>[2x]GVKSKAKKTVDKHSDEYKIRRE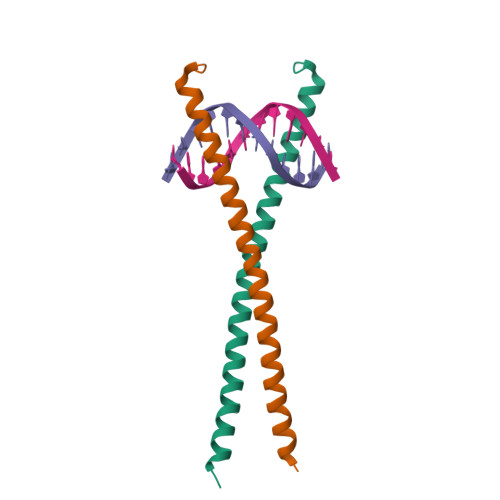RNNIAVRKSRDKAKMRNLETQHKVLELTAENERLQKKVEQLSRELSTLRNLFKQLPE>[4x]MAHHHHHHMNQFDVAVIGSGPGGYVAAIRCAQLGFKTVIIEKYSTLGGTCLNVGCIPSKALLDSSEHFENAKHTFATHGILIDEPKVDIAQMISRKNDVVDQTTKGINFLMDKNKITVLQGVGSFESATQIKVTKADGSSEVIEAKNTIIATGSKPSSLPFITLDKERVITSTEALNLKEVP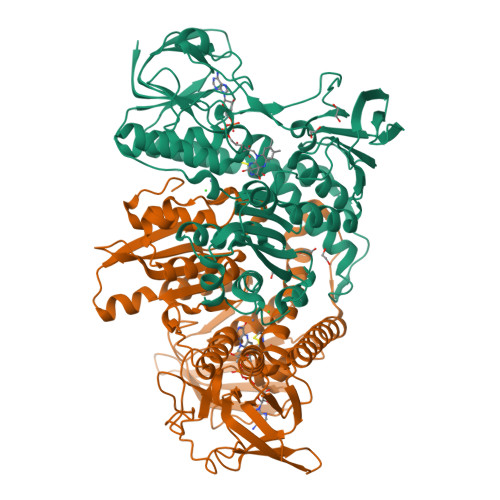KHLIVIGGGVIGLELGSVYLRLGSDVTVVEYLDKIIPGMDGTLSKELQKTLKKQGMKFMLSTAVSGVERNGDTVKVTAKDKKGEDVVVEGDYCLVSVGRRPYTDGLGLEKAGVELDERGRVKTNDHLQTNVPNIYAIGDVVKGAMLAHKAEEEGVFVAETLAGEKPHVNYNLIPGVVYTWPEVAGVGKTEEQLKEAGVAYKTGSFPMRALGRSRASMDTDGVIKILADEKTDEILGVHMIGARAADMIAEAVVAMEFRASAEDIARISHAHPTYTEAIKEAALDATGKRAIHM>GHMSTTTCTRFTDEYQLFEELGKGAFSVVRRCMKIPTGQEYAAKIINTKKLSARDHQKLEREARICRLLKHPNIVRLHDSISEEGFHYLVFDLVTGGELFEDIVAREYYSEADASHCIQQILESVNHCHLNGIVHRDLKPENLLLASKSKGAAV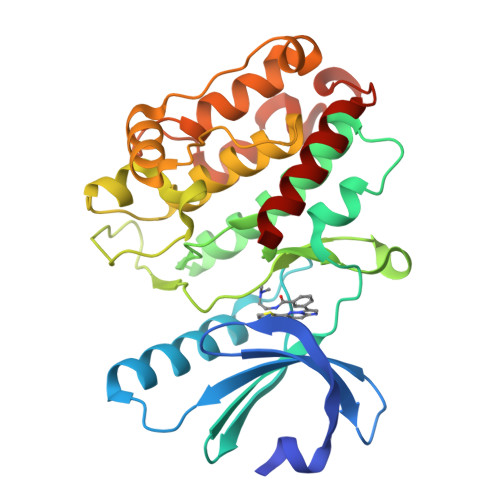KLADFGLAIEVQGDQQAWFGFAGTPGYLSPEVLRKDPYGKPVDMWACGVILYILLVGYPPFWDEDQHRLYQQIKAGAYDFPSPEWDTVTPEAKDLINKMLTINPAKRITASEALKHPWICQRSTVASMMHRQETVDCLKKFNARRKLK[2x]>[5x]GSGAMEKEEKSNLIYDKDPGYVWDNKNECEGAAEETYQELNYEPSISADKLTWTPTRLAKTVFNTYEDDDDFNVLCYFTDWSQYDPRIINKEIRDTGGRSADILRLNTPDGRPFKRLIYSFGGLIGDKKYSADGNASIAVRLGVATDPDDAIANHKGKTIPVDPDGAVLASINCGFTKWEAGDANERYNQEKAKGL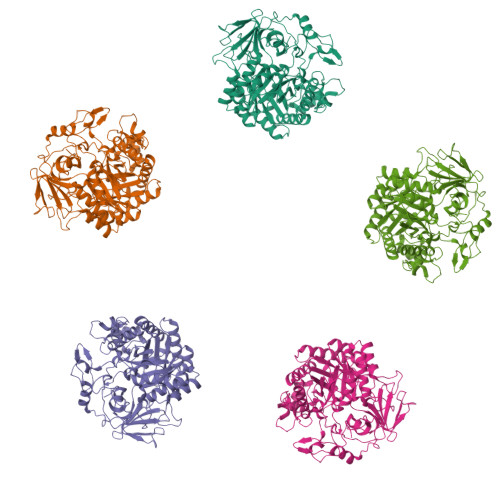LGGFRLLHEADKELEFSLSIGGWSMSGLFSEIAKDEILRTNFVEGIKDFFQRFPMFSHLDIDWEYPGSIGAGNPNSPDDGANFAILIQQITDAKISNLKGISIASSADPAKIDAANIPALMDAGVTGINLMTYDFFTLGDGKLSHHTNIYRDPSDVYSKYSIDDAVTHLIDEKKVDPKAIFIGYAGYTRNAKNATITTSIPSEEALKGTYTDANQTLGSFEYSVLEWTDIICHYMDFEKGEGRNGYKLVHDKVAKADYLYSEATKVFISLDTPRSVRDKGRYVKDKGLGGLFIWSGDQDNGILTNAAHEGLKRRIKNKVIDMTPFYLDSDEELPTYTEPAEPQCEACNIK> GAGCAGA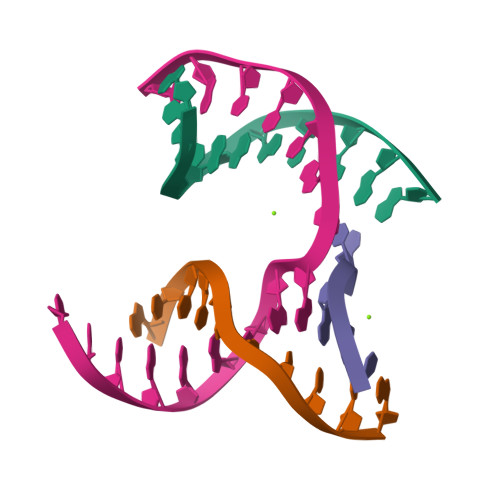CAAG;> ACTCCACTCA;> CTAGT;> TCTGAGTGGTGTCTGC>[2x]MHRTSNGSHATGGNLPDVASHYPVAYEQTLDGTVGFVIDEMTPERATASVEVTDTLRQRWGLVHGGAYCALAD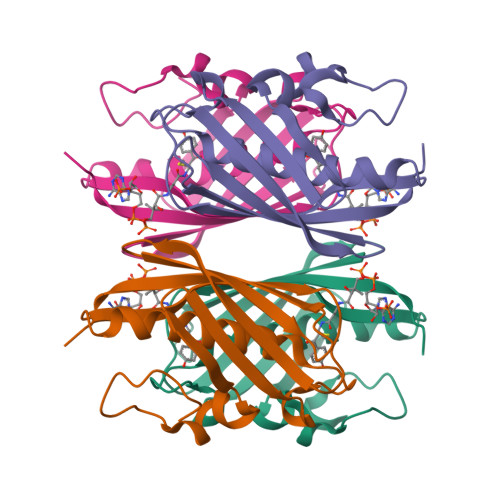MLATEATVAVVHEKGMMAVGQSNHTSFFRPVKEGHVRAEAVRIHAGSTTWFWDVSLRDDAGRLCAVSSMSIAVRPRRD>SNAMTQLTREQVLELFHQRSSTRYYDPAKKISDEDFECILECGRLSPSSVGSEPWKFLVIQNKTLREKMKPFSWGMINQLDNCSHLVVILAKKNARYDSPFFVDVMARKGLNAEQQQAALAKYKALQEEDMKLLENDRT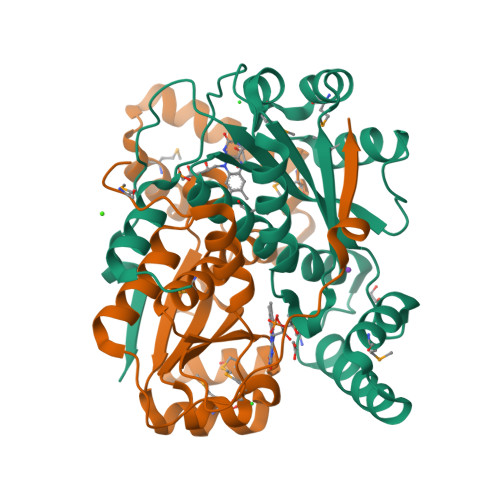LFDWCSKQTYIALANMLTGASALGIDSCPIEGFHYDKMNECLAEEGLFDPQEYAVSVAATFGYRSRDIAKKSRKGLDEVVRWVG[4x]>MGAAILPDLGTEILIPVCAVIGIAFALFQWLLVSKVKLSAVRDASPNAAAKNGYNDYLIEEEEGINDHNVVVKCAEIQNAISEGATSFLFTEYKYVGIFMVAFAILIFLFLGSVEGFSTSPQACSYDKTKTCKPALATAIFSTVSFLLGGVTSLVSGFLGMKIATYANARTTLEARKGVGKAFITAFRSGAVMGFLLAANGLLVLYIAINLFKIYYGDDWGGLFEAITGYGLGGSSMALFGRVGGGIYTKAADVGADLVGKVERNIPEDDPRNPAVIADNVGDNVGDIAGMGSDLFGSYAESSCAALVVASISSFGLNHELTAMLYPLIVSSVGILVCLLTTLFATDFFEIKAVKEIEPALKKQLVISTVLMTIGVAVVSFVALPTSFTIFNFGVQKDVKSWQLFLCVAVGLWAGLIIGFVTEYYTSNAYSPVQDVADSCRTGAATNVIFGLALGYKSVIIPIFAIAISIFVSFTFAAMYGIAVAALGMLSTIATGLAIDAYGPISDNAGGIAEMAGMSHRIRERTDALDAAGNTTAAIGKGFAIGSAALVSLALFGAFVSRASITTVDVLTPKVFIGLIVGAMLPYWFSAMTMKSVGSAALKMVEEVRRQFNTIPGLMEGTAKPDYATCVKISTDASIKEMIPPGALVMLTPLVVGILFGVETLSGVLAGSLVSGVQIAISASNTGGAWDNAKKYIEAGASEHARSLGPKGSDCHKAAVIGDTIGDPLKDTSGPSLNILIKLMAVESLVFAPFFATHGGLLFKIFSSHHHHHH[4x]

Membrane-bound pyrophosphatases (M-PPases) are enzymes that couple the synthesis or hydrolysis of pyrophosphate (PPi) to the vectorial transport of protons and/or sodium ions. In addition, M-PPases can be divided into seven functional classes on the basis of their monovalent cation binding (K+-dependent and K+-independent enzymes) and pumping specificity (H+-pumps (H+-PPases), Na+-pumps (Na+-PPases) and H+ and Na+ co-pumps (Na+/H+-PPases)) and on the placement of a ‘semi-conserved glutamate' essential for pumping activity. So far, the structures of two M-PPases have been solved in three different states: TmPPase in resting and product-bound states (TmPPase:Ca:Mg and TmPPase:Pi2, respectively)11 and VrPPase in a substrate-analogue imidodiphosphate (IDP)-bound state (VrPPase:IDP)12. These structures have shown that M-PPases are homodimers, with each protomer having 16 transmembrane helices (TMHs) and a vertically arranged, continuous active site structure with four distinctive parts: ‘hydrolytic centre', ‘coupling funnel', ‘ion gate' and ‘exit channel'3. In this article we present three structures: the Na+-pumping TmPPase with IDP and Na+ bound (TmPPase:IDP) at 3.5 Å resolution, the H+-pumping VrPPase with one phosphate bound (VrPPase:Pi) at 3.5 Å resolution, and the newly refined structure of TmPPase with the phosphate analogue, WO4 bound, at 4 Å resolution (TmPPase:WO4).

The overall structures of TmPPase:IDP, TmPPase:WO4 and VrPPase:Pi are similar to our previous structures with root mean squared deviation (r.m.s.d.) values of 0.7 Å for TmPPase:IDP-TmPPase:Pi2, 1.6 Å for TmPPase:IDP-TmPPase:Ca:Mg and 1.0 Å for VrPPase:Pi-VrPPase:IDP. In VrPPase:Pi, the extra Fo–Fc electron density in the PPi-binding pocket is a phosphate ion, just 0.6 Å from the leaving group phosphate in VrPPase:IDP. This phosphate ion is coordinated by K5.58, K16.38 and two Mg2+ ions, which are situated in a similar position to Mg2 and Mg3 in VrPPase:IDP and to the Ca2+ and Mg2+ in resting-state TmPPase. Notable was the volume of the hydrolytic centre, which approximately halves upon binding substrate: from 3,400 Å3 in resting-state TmPPase to 1,600 Å3 in the IDP-bound states of VrPPase and TmPPase, but expanding to 2,800 Å3 in VrPPase:Pi. The VrPPase:IDP has, instead of Na+, a number of water molecules lining the channel, including one coordinated by the gate residues. These water molecules are absent in the VrPPase:Pi, probably due to the low resolution of the structure (3.5 Å). Nonetheless, K16.50 is ordered in both states of VrPPase, unlike in TmPPase.3-(2-(6-AMINO-4-METHYLPYRIDIN-2-YL)ETHYL)-5-(METHYL(2-(METHYLAMINO)ETHYL)AMINO)BENZONITRILE | 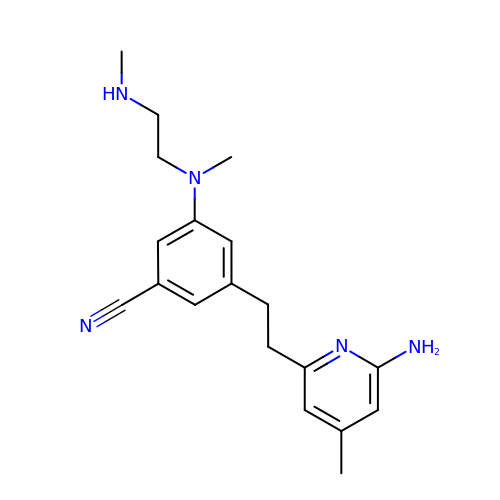C19 H25 N5 | RYFZEWNGJTVNMY-UHFFFAOYSA-N>[2x]SMTESTVDRINGITPSALDLIGNTPLIALDRLWPGPGRLLAKCEFLNPTASLKDRSSYYMIAKAKESGQLKDGESVIEVTSGNQGGGIACVTAVMGHPFTVTMSKGNSPQRAIMMNA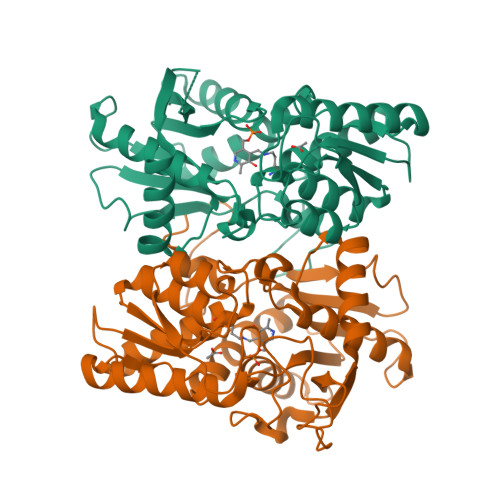LGANVILVDQVTGKPGNVTADDVAAAEETAMKIREETNAYYVDQFNNPTNCLAHYETTGPEIWRQTNGRIDAFLVGCGTGGCFVGTSKFLKEKNPNVRCFVVEPEGCQPIAGCTITKPLHLLQGSGYGCVPTLFDKKVYNDSISVSDEEAIEYRKLLGQKEGLFCGFTTGGNIAAAIKLLKSGQLPKDAWVVTILCDSGLKYPE2-(3-fluorophenyl)quinoline-4-carboxylic acid | C16 H10 F 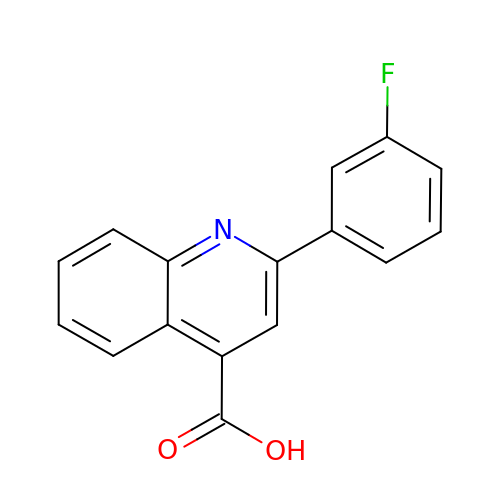N O2 | PCKQJQMHOYYDMQ-UHFFFAOYSA-N>[2x]MGSSHHHHHHSSGMVFYFTSSSVNSSAY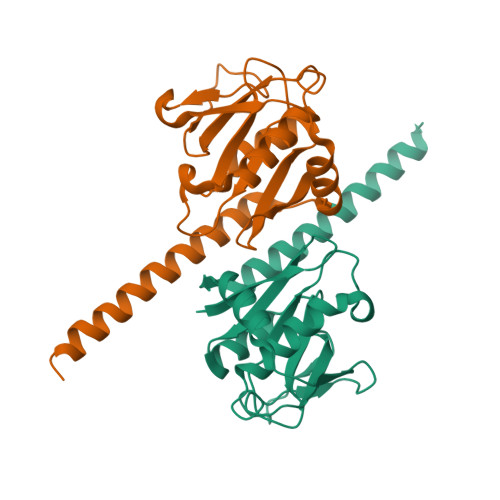TIYMGKDKYENEDLIKHGWPEDIWFHVDKLSSAHVYLRLHKGENIEDIPKEVLMDCAHLVKANSIQGCKMNNVNVVYTPWSNLKKTADMDVGQIGFHRQKDVKIVTVEKKVNEILNRLEKTKVERFPDLAAEKECRDREERNEKKAQIQEMKKREKEEMKKKREM Faithful chromosome segregation requires robust, load-bearing attachments of chromosomes to the mitotic spindle, a function accomplished by large macromolecular complexes termed kinetochores. In most eukaryotes, the constitutive centromere-associated network (CCAN) complex of the inner kinetochore recruits to centromeres the ten-subunit outer kinetochore KMN network that comprises the KNL1C, MIS12C and NDC80C complexes. The KMN network directly attaches CCAN to microtubules through MIS12C and NDC80C. The outer kinetochore is made up of the central and evolutionarily conserved ten-subunit KMN network complex, comprising the MIS12 (Mis12, Dsn1, Nsl1, Pmf1), NDC80 (Ndc80, Nuf2, Spc24, Spc25) and KNL1 (Knl1, ZWINT) complexes as well as auxiliary microtubule-associated components, such as the SKA complex, that vary between species.

We subjected the reconstituted KMN network to cryo-EM analysis and obtained a 3.0-Å-resolution reconstruction of the KMN network junction (KMNJunction) containing complete MIS12C, Spc24–Spc25 and all folded domains of KNL1C. The only components that we did not observe at high resolution were the Ndc80 and Nuf2 proteins, which seem to be flexibly connected to Spc24–Spc25 at the tetramerization junction. At the core of the KMNJunction complex is MIS12C, which comprises a tetrameric coiled coil connected to two head domains (MIS12CHead-1 and MIS12CHead-2). A salient feature of KMNJunction is the coiled coils of Spc24–Spc25 and Knl1–ZWINT that run perfectly parallel to one another, giving the entire assembly a prong-like shape. The Spc24–Spc25RWD and Knl1RWD domains are rigidly docked onto the top of the MIS12C stalk, and their interactions with MIS12C are further stabilized by extensive peptide interactions with the C termini of the MIS12C subunits Dsn1 and Nsl1. Knl1RWD-C rigidly docks and recognizes a shallow surface formed by the Dsn1 and Pmf1 coiled coils, whereas Knl1RWD-N uses a canonical RWD protein-interaction groove to bind the otherwise disordered Nsl1 C-terminal tail. Overall, Nsl1 uses two highly conserved motifs at its C terminus to bind to the Knl1–ZWINT complex: a YPLR motif binds to Knl1RWD-N, and a VLKRK motif binds across the Knl1–ZWINT coiled coil. In our reconstruction, MIS12CHead-2 directly contacts MIS12CHead-1, resulting in an auto-inhibited MIS12C state. This state is stabilized by the Dsn1N auto-inhibitory segment (residues 93–113), which forms two contacts with MIS12CHead-1: (1) a linchpin formed by the WRR motif (residues 96–98) of Dsn1N, which locks into the hydrophobic pocket at the Mis12–Pmf1 interface and connects Mis12–Pmf1 to the coiled-coil connector-α3 helices of Dsn1–Nsl1; and (2) a zipper-like interaction of the RKSL motif (residues 107–110) that bridges MIS12CHead-1 and MIS12CHead-2 through both electrostatic and non-polar interactions.

> MTSVTRSEIIDEKGPVMSKTHDHQLESSLSPVEVFAKTSASLEMNQGVSEERIHLGSSPKKGGNCDLSHQERLQSKSLHLSPQEQSASYQDRRQSWRRASMKETNRRKSLHPIHQGITELSRSISVDLAESKRLGCLLLSSFQFSIQKLEPFLRDTKGFSLESFRAKASSLSEELKHFADGLETDGTLQKCFEDSNGKASDFSLEASVAEMKEYITKFSLERQTWDQLLLHYQQEAKEILSRGSTEAKITEVKVEPMTYLGSSQNEVLNTKPDYQKILQNQSKVFDCMELVMDELQGSVKQLQAFMDESTQCFQKVSVQLGKRSMQQLDPSPARKLLKLQLQNPPAIHGSGSGSCQ;> MAAFRDIEEVSQGLLSLLGANRAEAQQRRLLGRHEQVVERLLETQDGAEKQLREILTMEKEVAQSLLNAKEQVHQGGVELQQLEAGLQEAGEEDTRLKASLLQLTRELEELKEIEADLERQEKEVDEDTTVTIPSAVYVAQLYHQVSKIEWDYECEPGMVKGIHHGPSVAQPIHLDSTQLSRKFISDYLWSLVDTEW;> MVEDELALFDKSINEFWNKFKSTDTSCQMAGLRDTYKDSIKAFAEKLSVKLKEEERMVEMFLEYQNQISRQNKLIQEKKDNLLKLIAEVKGKKQELEVLTANIQDLKEEYSRKKETISTANKANAERLKRLQKSADLYKDRLGLEIRKIYGEKLQFIFTNIDPKNPESPFMFSLHLNEARDYEVSDSAPHLEGLAEFQENVRKTNNFSAFLANVRKAFTATVYN;> MDGVSSEANEENDNIERPVRRRHSSILKPPRSPLQDLRGGNERVQESNALRNKKNSRRVSFADTIKVFQTESHMKIVRKSEMEGCSAMVPSQLQLLPPGFKRFSCLSLPETETGENLLLIQNKKLEDNYCEITGMNTLLSAPIHTQMQQKEFSIIEHTRERKHANDQTVIFSDENQMDLTSSHTVMITKGLLDNPISEKSTKIDTTSFLANLKLHTEDSRMKKEVNFSVDQNTSSENKIDFNDFIKRLKTGKCSAFPDVPDKENFEIPIYSKEPNSASSTHQMHVSLKEDENNSNITRLFREKDDGMNFTQCHTANIQTLIPTSSETNSRESKGNDITIYGNDFMDLTFNHTLQILPATGNFSEIENQTQNAMDVTTGYGTKASGNKTVFKSKQNTAFQDLSINSADKIHITRSHIMGAETHIVSQTCNQDARILAMTPESIYSNPSIQGCKTVFYSSCNDAMEMTKCLSNMREEKNLLKHDSNYAKMYCNPDAMSSLTEKTIYSGEENMDITKSHTVAIDNQIFKQDQSNVQIAAAPTPEKEMMLQNLMTTSEDGKMNVNCNSVPHVSKERIQQSLSNPLSISLTDRKTELLSGENMDLTESHTSNLGSQVPLAAYNLAPESTSESHSQSKSSSDECEEITKSRNEPFQRSDIIAKNSLTDTWNKDKDWVLKILPYLDKDSPQSADCNQEIATSHNIVYCGGVLDKQITNRNTVSWEQSLFSTTKPLFSSGQFSMKNHDTAISSHTVKSVLGQNSKLAEPLRKSLSNPTPDYCHDKMIICSEEEQNMDLTKSHTVVIGFGPSELQELGKTNLEHTTGQLTTMNRQIAVKVEKCGKSPIEKSGVLKSNCIMDVLEDESVQKPKFPKEKQNVKIWGRKSVGGPKIDKTIVFSEDDKNDMDITKSYTIEINHRPLLEKRDCHLVPLAGTSETILYTCRQDDMEITRSHTTALECKTVSPDEITTRPMDKTVVFVDNHVELEMTESHTVFIDYQEKERTDRPNFELSQRKSLGTPTVICTPTEESVFFPGNGESDRLVANDSQLTPLEEWSNNRGPVEVADNMELSKSATCKNIKDVQSPGFLNEPLSSKSQRRKSLKLKNDKTIVFSENHKNDMDITQSCMVEIDNESALEDKEDFHLAGASKTILYSCGQDDMEITRSHTTALECKTLLPNEIAIRPMDKTVLFTDNYSDLEVTDSHTVFIDCQATEKILEENPKFGIGKGKNLGVSFPKDNSCVQEIAEKQALAVGNKIVLHTEQKQQLFAATNRTTNEIIKFHSAAMDEKVIGKVVDQACTLEKAQVESCQLNNRDRRNVDFTSSHATAVCGSSDNYSCLPNVISCTDNLEGSAMLLCDKDEEKANYCPVQNDLAYANDFASEYYLESEGQPLSAPCPLLEKEEVIQTSTKGQLDCVITLHKDQDLIKDPRNLLANQTLVYSQDLGEMTKLNSKRVSFKLPKDQMKVYVDDIYVIPQPHFSTDQPPLPKKGQSSINKEEVILSKAGNKSLNIIENSSAPICENKPKILNSEEWFAAACKKELKENIQTTNYNTALDFHSNSDVTKQVIQTHVNAGEAPDPVITSNVPCFHSIKPNLNNLNGKTGEFLAFQTVHLPPLPEQLLELGNKAHNDMHIVQATEIHNINIISSNAKDSRDEENKKSHNGAETTSLPPKTVFKDKVRRCSLGIFLPRLPNKRNCSVTGIDDLEQIPADTTDINHLETQPVSSKDSGIGSVAGKLNLSPSQYINEENLPVYPDEINSSDSINIETEEKALIETYQKEISPYENKMGKTCNSQKRTWVQEEEDIHKEKKIRKNEIKFSDTTQDREIFDHHTEEDIDKSANSVLIKNLSRTPSSCSSSLDSIKADGTSLDFSTYRSSQMESQFLRDTICEESLREKLQDGRITIREFFILLQVHILIQKPRQSNLPGNFTVNTPPTPEDLMLSQYVYRPKIQIYREDCEARRQKIEELKLSASNQDKLLVDINKNLWEKMRHCSDKELKAFGIYLNKIKSCFTKMTKVFTHQGKVALYGKLVQSAQNEREKLQIKIDEMDKILKKIDNCLTEMETETKNLEDEEKNNPVEEWDSEMRAAEKELEQLKTEEEELQRNLLELEVQKEQTLAQIDFMQKQRNRTEELLDQLSLSEWDVVEWSDDQAVFTFVYDTIQLTITFEESVVGFPFLDKRYRKIVDVNFQSLLDEDQAPPSSLLVHKLIFQYVEEKESWKKTCTTQHQLPKMLEEFSLVVHHCRLLGEEIEYLKRWGPNYNLMNIDINNNELRLLFSSSAAFAKFEITLFLSAYYPSVPLPSTIQNHVGNTSQDDIATILSKVPLENNYLKNVVKQIYQDLFQDCHFYH;> MSVDPMTYEAQFFGFTPQTCMLRIYIAFQDYLFEVMQAVEQVILKKLDGIPDCDISPVQIRKCTEKFLCFMKGHFDNLFSKMEQLFLQLILRIPSNILLPEDKCKETPYSEEDFQHLQKEIEQLQEKYKTELCTKQALLAELEEQKIVQAKLKQTLTFFDELHNVGRDHGTSDFRESLVSLVQNSRKLQNIRDNVEKESKRLKIS;> MAGSPELVVLDPPWDKELAAGTESQALVSATPREDFRVRCTSKRAVTEMLQLCGRFVQKLGDALPEEIREPALRDAQWTFESAVQENISINGQAWQEASDNCFMDSDIKVLEDQFDEIIVDIATKRKQYPRKILECVIKTIKAKQEILKQYHPVVHPLDLKYDPDPAPHMENLKCRGETVAKEISEAMKSLPALIEQGEGFSQVLRMQPVIHLQRIHQEVFSSCHRKPDAKPENFITQIETTPTETASRKTSDMVLKRKQTKDCPQRKWYPLRPKKINLDT;> MAEASSANLGSGCEEKRHEGSSSESVPPGTTISRVKLLDTMVDTFLQKLVAAGSYQRFTDCYKCFYQLQPAMTQQIYDKFIAQLQTSIREEISDIKEEGNLEAVLNALDKIVEEGKVRKEPAWRPSGIPEKDLHSVMAPYFLQQRDTLRRHVQKQEAENQQLADAVLAGRRQVEELQLQVQAQQQAWQALHREQRELVAVLREPE;> MEAAETEAEAAALEVLAEVAGILEPVGLQEEAELPAKILVEFVVDSQKKDKLLCSQLQVADFLQNILAQEDTAKGLDPLASEDTSRQKAIAAKEQWKELKATYREHVEAIKIGLTKALTQMEEAQRKRTQLREAFEQLQAKKQMAMEKRRAVQNQWQLQQEKHLQHLAEVSAEVRERKTGTQQELDRVFQKLGNLKQQAEQERDKLQRYQTFLQLLYTLQGKLLFPEAEAEAENLPDDKPQQPTRPQEQSTGDTMGRDPGVSFKAVGLQPAGDVNLP> MDEALIKDYHSIREQIDQYTKDMVLVMQHPTNCVKYINPGRLMHVVTSDGTDFGWGVIINFYERRPERNNPNPGWSPQESYVVEVLLRLSSDSGSVDSKLKDNQCIPAGIAPVTQKNDPGRWEVVPCLLSCMHGLSQIK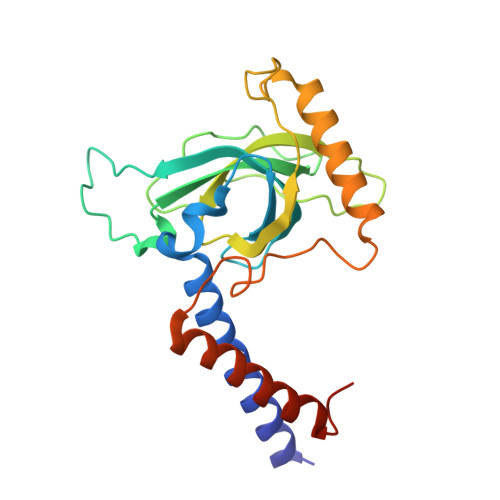LHVPDKKSGGSMDDPETRRRVGKSLLEVQRRFEDGIPHMDPIENMHIRDVEFKKLLRKIEVLESRLVANPLHNSGGSGGS>SMLWVGVVSIFPEMFRAISDYGITSRAVKQGLLTLTCWNPRVYTEDRHQTVDDRPFGGGPGMVMKIKPLEGALADARQAAGGRKAKVIYLSPQGRQLTQAGVRELAEEEALILIAGRYEGIDERFIEEHVDEEWSIGDYVLSGGELPAMVLVDAVTRLLPGALGHADSAEEDSFTDGLLDCPHYTRPEVYADKRVPEVLLSGNHE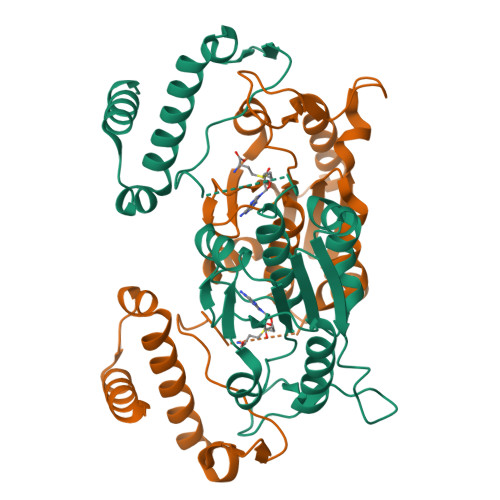HIRRWRLQQALGRTWERRADLLDSRSLSGEEQKLLAEYIRQRD[2x]> MEYAEHQGRIKNAREAHSQIEKRRRDKMNSFIDELASLVPTCNAMSRKLDKLTVLRMAVQHMKTLRGATNPYTEANYKPTFLSDDELKHLILRAADGFLFVVGCDRGKILFVSESVFKILNYSQNDLIGQSLFDYLHPKDIAKVKEQLSSSDTAPRERLIDAKTGLPVKTDITPGPSRLCSGARRSFFCRMKCNRPSVKVEDKDFASTCSKKKADRKSFCTIHSTGYLKSWPPTKMGLDEDNEPDNEGCN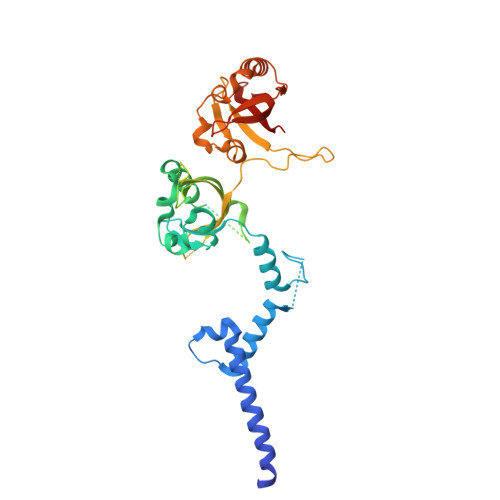LSCLVAIGRLHSHMVPQPANGEIRVKSMEYVSRHAIDGKFVFVDQRATAILAYLPQELLGTSCYEYFHQDDIGHLAECHRQVLQTREKITTNCYKFKIKDGSFITLRSRWFSFMNPWTKEVEYIVSTNTVVLANVLE> ACDYTCGSNCYSSSDVSTAQAAGYKLHEDGETVGSNSYPHKANNYEGFAFSVSSPYYEWPILSSGDVYSGGSPGADRVVFNENNQLAGVITHT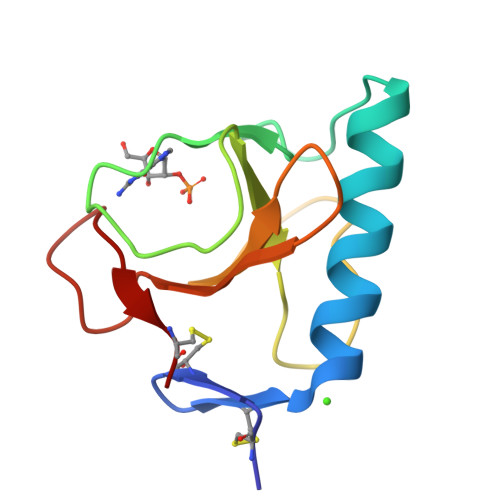GASGNNFVECT> GNDLLEPKVYFESKEYNFSVEDEMDVMTFDLVSRLSSATSSQVDVSYSVAEPSVVDEYNAKYGTNYEMLDVSQVKLSSTTSSISSGKLYADNIEVELSGLEALKAGNSYVLPMRVHSSSVSTLSGTNIAYFFFSKPLKITKAGNFSNHYISVKFPVGTFFSSFTYEALINVDYFLDNNTIMGTEGVMILRIGDAGGGITPKDYLEVAGGQNYRVTKPLLTNRWYHVALTYDQPTGKTGIYVNGEK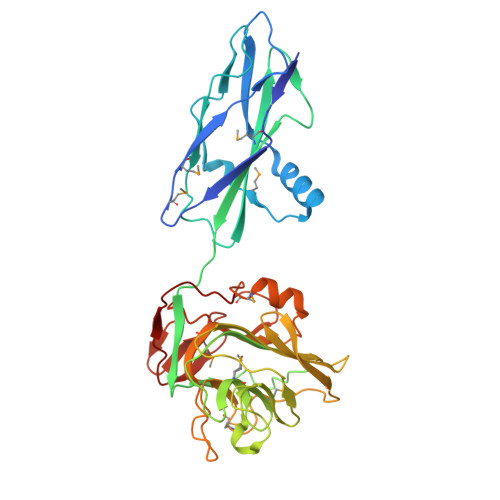WAGSDWGIDGFDPNSDMGFYIGRIYGFKWGERPFHGKMSEVRVWSVARTENQLKQNMLGVDPASEGLALYYKLDGSETQEGGVIKDATGRINGTTNGITIKTLDAPIAIN> KIPSKETPRGVAIAEPIIVEHSVDLLMVGGGMGNCGAAFEAVRWADKYAPEAKILLVDKASLERSGAVAQGLSAINTYLGDNNADDYVRMVRTDLMGLVREDLIYDLGRHVDDSVHLFEEWGLPVWIKDEHGHNLDGAQAKAAGKSLRNGDKPVRSGRWQIMINGESYKVIVAEAAKNALGQDRIIERIFIVKLLLDKNTPNRIAGAVGFNLRANEVHIFKANAMVVACGGAVNVYRPRSVGEGMGRAWYPVWNAGSTYTMCAQVGAEMTMMENRFVPARFKDGYGPVGAWFLLFKAKATNCKGEDYCATNRAMLKPYEERGYAKGHVIPTCLRNHMMLREMREGRGPIYMDTKTALQTSFATMSPAQQKHLEAEAWEDFLDMCVGQANLWAATNCAPEERGSEIMPTEPYLLGSHSGCCGIWASGPDEAWVPEDYKVRAANGKVYNRMTTVEGLWTCADGVGASGHKFSSGSHAEGRIVGKQMVRWYLDHKDFKPEFVETAEELKTLIYRPYYNYEKGKGA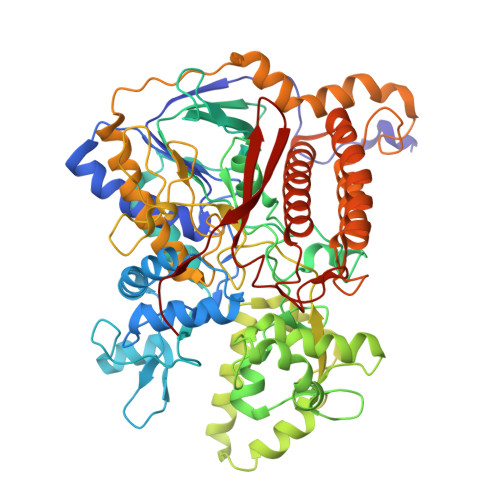STCPVVNPEYISPKNFMMRLIKCTDEYGGGVGTYYNTSKALLDTGFWLMEMLEEDSLKLAARDLHELLRCWENYHRLWTVRLHMQHIAFREESRYPGFYYRADFLGLDDSKWKCFVNSKYDPAKKETKIFKKPYYQIIPD> MDINIDDILAELDKETTAVDSTKITQGSSSTTHRDANTIVGSSLDLNDKTQIYVSPQQDFSDLMKSWKNERCSPELLPYPHQLMKRLLNRISMQSQLIENISMGFLDMQNASNANPPMPNESKLPLLCMETELERLKFVIRSYIRCRLSKIDKFSLYLRQLNEDENSLISLTDLLSKDEIKYHDTHSLIWLKLVNDSILKYMPEELQAINDTEGSVNMIDEPDWNKFVFIHVNGPPDGKWNEDPLLQENEFGKPCYTVTIPDLKEEVELTIGSI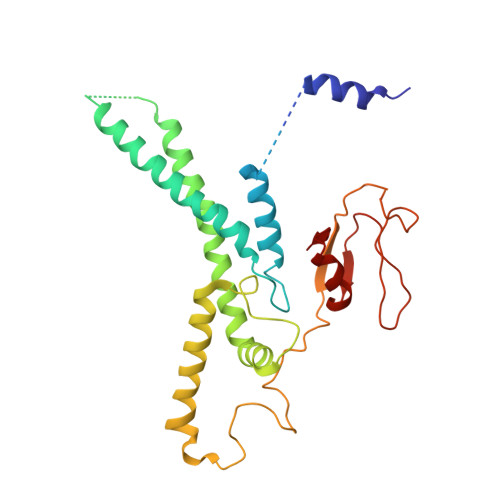YVMRYEVIRDLLRDDKVALI>MSLKKKIAVVTGATGGMGIEIVKDLSRDHIVYALGRNPEHLAALAEIEGVEPIESDIVKEVLEEGGVDKLKNLDHVDTLVHAAAVARDTTIEAGSVAEWHAHLDLNVIVPAELSRQLLPALRAASGCVIYINSGAGNGPHPGNTIYAASKHALRGLADAFRKEEANNGIRVSTVSPGPTNTPMLQ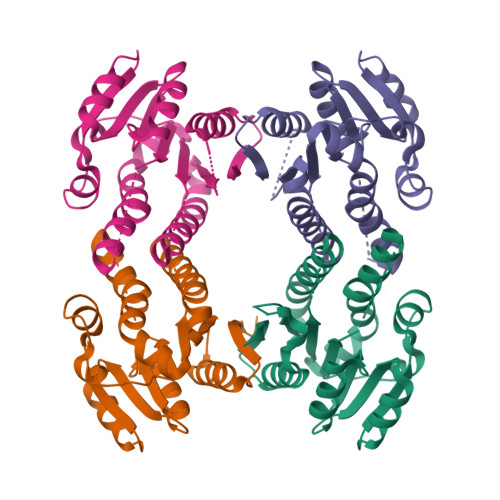GLMDSQGTNFRPEIYIEPKEIANAIRFVIDAGETTQITNVDVRPRIELADRKEGHHHHHH[8x]>[2x]MQSPPPDPLGDCLRNWEDLQQDFQGIQETHRLYRLKLEELTKLQANCTNSITRQKKRLQELALVLKKCRPSLPSESMEAAQELENQMKERQGLFFDMEAYLPKKNGLYLSLVLGNVNVTLLSKQAKFAYKDEYEKFKLYLTIILIVISFTCRFLLNSRVTDAAFNFLLVWYYCTLTIRESILINNGSRIKGWWVFHHYVSTFLSGVMLTWPDGLMYQKFRNQFLSFSMYQSFVQFLQYYYQSGCLYRLRALGERHTMDLTVEGFQSWMWRGLTFLLPFLFFGHFWQLFNALTLFNLARDPECKEWQVLMCGFPFLLLFLGNFFTTLRVVHQKFHSQQHGNKKD

TACAN, originally identified in a proteomics screen and called TMEM120A, was categorized as a nuclear envelope protein (NET29) that participates in lipid metabolism. TACAN is an α-helical TM protein that forms a symmetric dimer. Each protomer consists of six TM helices (S1–S6), which form a barrel surrounding a tunnel open to the cytoplasm. The TACAN protomer is related in three-dimensional structure to a fatty acid elongase, ELOVL7.

Alongside the functional characterization, we analyzed the structure of TACAN determined at 3.5 Å resolution using single-particle cryo-EM. The two protomers of the TACAN dimer bury an extensive surface area of 3049 Å2, mediated through the TM domain as well as two long N-terminal helices that form a coiled coil. Non-continuous density was observed inside the tunnel, suggesting the presence of a small, non-protein molecule. The TM domain in TACAN is indeed similar to ELOVL7. TACAN conserves two of the four histidine residues. In the purified TACANWT sample, the apo form is dominant and incubation with S-ethyl-CoA shifts it to one and two analogue bound forms. In addition, no enzymatic activity was observed for TACAN using a free-CoA detection assay (for details), which demonstrated robust activity for ELOVL7, thus TACAN does not appear to catalyze the same reaction as ELOVL7. In conclusion, we do not find evidence that TACAN is a mechanosensitive ion channel.[(2R,4S,6R)-4-azanyl-4,6-dimethyl-5,5-bis(oxidanyl)oxan-2-yl] 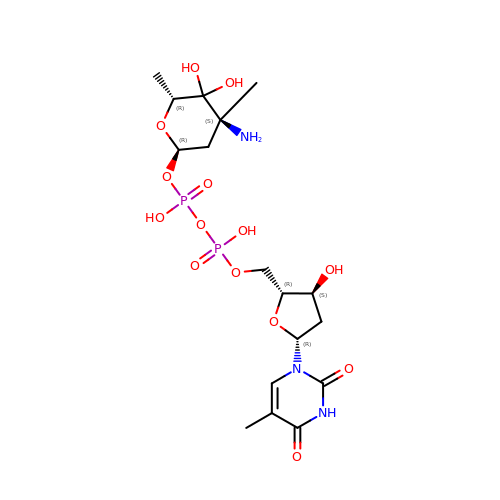[[(2R,3S,5R)-5-[5-methyl-2,4-bis(oxidanylidene)pyrimidin-1-yl]-3-oxidanyl-oxolan-2-yl]methoxy-oxidanyl-phosphoryl] hydrogen phosphate | C17 H29 N3 O14 P2 | GACNZVKWDHTCBB-HHMBNNFFSA-N>MEKVREIVREGIRVGNEDPRRIIHAFKVGLALVLVSSFYYYQPFGPFTDYFGINAMWAVMTVVVVFEFSVGATLGKGLNRGVATLVAGGLGIGAHQLARLSGATVEPILLVMLVFVQAALSTFVRFFPWVKTKFDYGILIFILTFALISLSGFRDEEIMDLAESRLSTVVIGGVSCILISIFVCPVWAGQDLHSLLASNFDTLSHFLQDFGDEYFEAREKGDYKVVEKRKKNLERYKSVLDSKSDEEALANYAEWEPPHGQFRFRHPW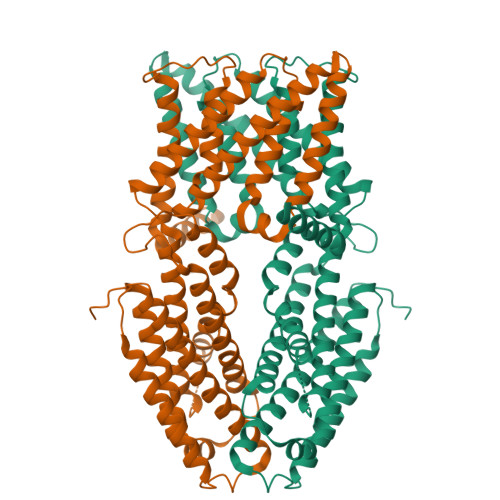KQYVAVGALLRQCAYRIDALNSYINSDFQIPVDIKKKLETPLRRMSSESGNSMKEMSISLKQMIKSSSSDIHVSNSQAACKSLSTLLKSGILNDVEPLQMISLMTTVSMLIDIVNLTEKISESVHELASAARFKNKMRPTVLYEKSDSGSIGRAMPIDSHEDHHVVTVLHDVDNDRSNNVDDSRGGSSQDSCHHVAIKIVDDNSNHEKHEDGEIHVHTLSNGHLQLEGGSSGGWSHPQFEK[2x]Mature CVB1 virions, like other enteroviruses, have 4 structural proteins termed viral protein 1–4 (VP1–4). They form an icosahedrally-symmetric capsid of about 30 nm in diameter with VP1 around the 5-fold, VP2 on the sides of the 2-fold and alternating VP2 and VP3 around 3-fold symmetry axes. At the base of VP1, there is a hydrophobic pocket which normally contains a lipid factor. Similar to empty particles, recombinantly produced Virus-Like Particles (VLPs) closely mimic the structure of infectious virions but lack genetic material.

Through cryoEM and single-particle image processing, two distinct particle populations were separated. These particle populations were termed compact and expanded, structurally corresponding to mature native CVB1 virions and CVB1 A-particles respectively. Particle sets were processed in cryoEM and Scipion to 2.15 Å resolution reaching Nyqvist. The structure and position of VP0 in VLPs corresponds to VP2 and VP4 in mature virions, however lacking a 39 residues long section on the inside of the capsid and missing an N-terminus and myristoyl group. Furthermore, N-terminus arms embracing the VP4 in the native CVB1 could not be modelled prior to residue 56 in the CVB1-VLPTween80. Other characteristic structural features of native CVB1 are seen, such as the VP1 around the 5-fold, lipid factor inside the hydrophobic pocket, VP0 helices on the sides of the 2-fold symmetry axis and VP0 and VP3 alternating around a 3-fold. At the current resolution, an ion coordinated between three D203 at the 3-fold can be observed in both expanded and compact forms. In the expanded CVB1-VLPsTween80, a forked density is present above cysteins which could be additional ion densities and in the compact CVB1-VLPTween80 two conformations of VP3 R232 are resolved. Here we observed two structural differences of CVB1-VLPsTween80 compared to native CVB1 which are the presence of a VP3 loop in the pore of the expanded CVB1-VLPsTween80 and an additional density in the interprotomer pocket of compact CVB1-VLPTween80. Despite the lower immunizing properties, VLPs have shown to be stable for at least one month and can handle freezing and thawing while retaining almost 50% of the particles in the compact form.

> YHSRSESSIENFLCRAACVYYATYTNNSEKGYAEWVINTRQVAQLRRKLELFTYLRFDLELTFVITSAQQPSTATSVDAPVQTHQIMYVPPGGPVPTKVTDYAWQTSTNPSVFWTEGNAPPRMSIPFISIGNAYSCFYDGWTQFSRNGVYGINTLNNMGTLYMRHVNEAGQGPIKSTVRIYFKPKHVKAWVPRPPRLCQYEKQKNVNFTPTGVTTTRVGITTT;> VRSITLGNSTITTQECANVVVGYGVWPEYLKDNEATAEDQPTQPDVATCRFYTLESVQWMKNSAGWWWKLPDALSQMGLFGQNMQYHYLGRTGYTIHVQCNASKFHQGCLLVVCVPEAEMGCSNLNNTPEFAELSGGDTARMFTDTQIGETNSKKVQTAVWNAGMGVGVGNLTIYPHQWINLRTNNSATIVMPYINSVPMDNMFRHNNLTLMIIPFVPLNYSEGSSPYVPITVTIAPMCAEYNGLRLASSQ;> GLPVMTTPGSTQFLTSDDFQSPSAMPQFDVTPEMQIPGRVNNLMEIAEVDSVVPVNNTEANVNSLKAYQIPVQSNSDNGKQVFGFPLQPGANGVLNRTLLGEILNYYTHWSGSIKLTFMFCGSAMATGKFLLAYSPPGAGVPKNRKDAMLGTHVIWDVGLQSSCVLCVPWISQTHYRYVVEDEYTAAGYITCWYQTNIVVPADVQSSCDILCFVSACNDFSVRMLKDTPFIRQDTFYQ;> YTNINYYKDAASNSANR> MSEPGAGPSDGQVVTRKIRLHKVMRPLDESSPSSQEQHMDRRLAEILPAIADLPVPGPSGAGGSPADARAVEMRRLRGTQQELAQMEAMELATLFDMSKPHP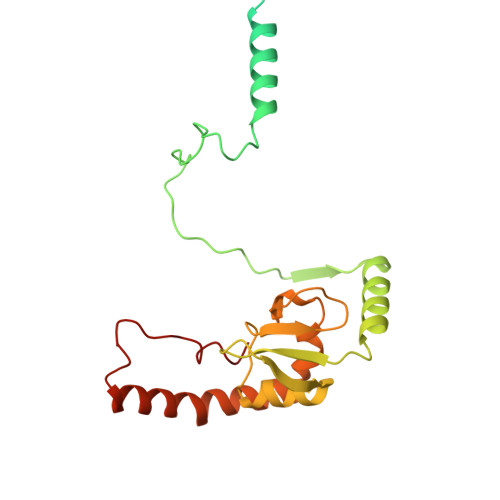LDNAAPATPWKGELRPVPRKIVLSPYQYEMINYQRMLMRKNIWYYRDRMNVPRGPCPLHVVKEAWVSGIVDENTLFWGHGLYDWLPAKNIKLLLPMVRTPEVRFATWIKRTFSLKPSLNRIREQRKEHRDPQEASLQVELMR> HKCDITLQEIIKDLNSLTEQKTLCTELTVTDIFAASKNTTEKETFC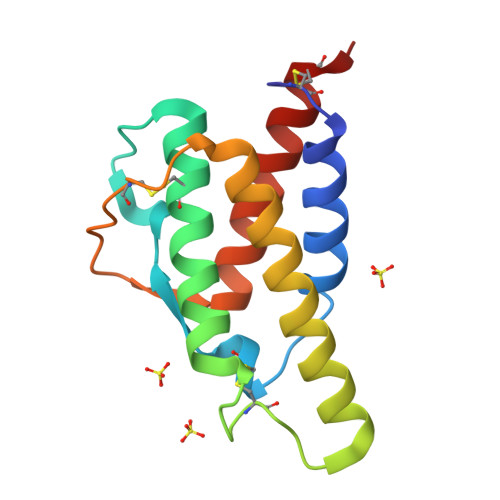RAATVLRQFYSHHEKDTRCLGATAQQFHRHKQLIRFLKRLDRNLWGLAGLNSCPVKEANQSTLENFLERLKTIMREKYSKCSS>GSWSVKELEDKNEELLSEIAHLKNEVARLKKLLQRCLAANQELRDAMRQSNQILRERAEELLHFQASQREEKEFLMS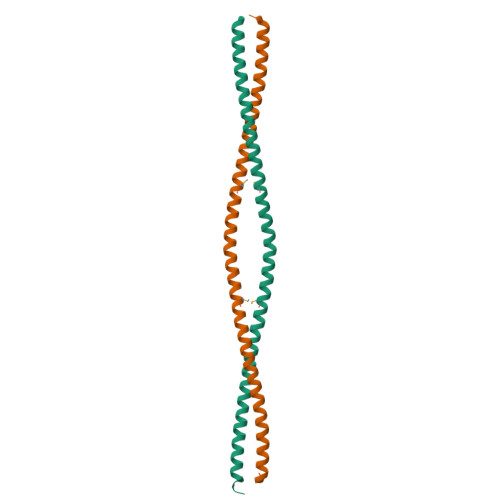KFQEARKLVERLGLEKLELEDKNEELLSEIAHLKNEVARLKKLVGER[2x]>[2x]MRLLTALFAYFIVALILAFSVSAKSMH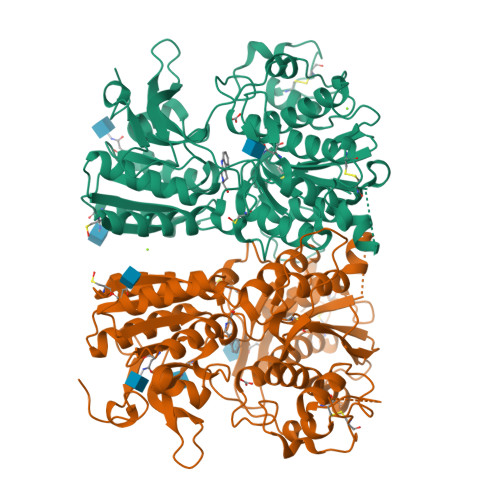HHHHHHHSAWSHPQFEKEFYGPDQRAQKKGDIILGGLFPIHFGVAAKDQDLKSRPESVECIRYNFRGFRWLQAMIFAIEEINSSPALLPNLTLGYRIFDTCNTVSKALEATLSFVAQNKIDSLNLDEFCNCSEHIPSTIAVVGATGSGVSTAVANLLGLFYIPQVSYASSSRLLSNKNQFKSFLRTIPNDEHQATAMADIIEYFRWNWVGTIAADDDYGRPGIEKFREEAEERDICIDFSELISQYSDEEEIQHVVEVIQNSTAKVIVVFSSGPDLEPLIKEIVRRNITGKIWLASEAWASSSLIAMPQYFHVVGGTIGFALKAGQIPGFREFLKKVHPRKSVHNGFAKEFWEETFNCHLQEGAKGPLPVDTFLRGHEESGDRFSNSSTAFRPLCTGDENISSVETPYIDYTHLRISYNVYLAVYSIAHALQDIYTCLPGRGLFTNGSCADIKKVEAWQVLKHLRHLNFTNNMGEQVTFDECGDLVGNYSIINWHLSPEDGSIVFKEVGYYNVYAKKGERLFINEEKILWSGFSREVPFSN>[2x]TSNFFCGEPIDYRGITAHRLVGAEPRPPVSGTRYAKVPGVPDEYKTGYRPANLGRSDPDSDKSLMNIAVKNLQVYQQEPKLDKVDEFIERAAADVLGYLRFLTKGERQANLNFKAAFNTLDLSTSCGPFVPGKKIDHVKDGVMDQVLAKHLYKCWSVANSGKALHHIYACGLKDELRPLDKVKEGKKRLLWGCDVGVAVCAAAVFHNICYKLKMVARFGPIAVGVDMTSRDVDVIINNLTSKASDFLCLDYSKWDSTMSPCVVRLAIDILADCCEQTELTKSVVLTLKSHPMTILDAMIVQTKRG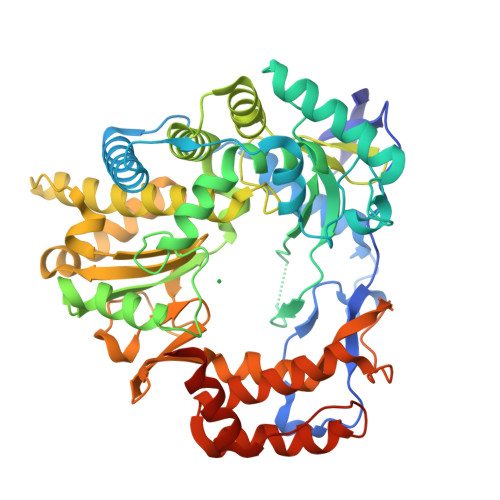LPSGMPFTSVINSICHWLLWSAAVYKSCAEIGLHCSNLYEDAPFYTYGDDGVYAMTPMMVSLLPAIIENLRDYGLSPTAADKTEFIDVCPLNKISFLKRTFELTDIGWVSKLDKSSILRQLEWSKTTSRHMVIEETYDLAKEERGVQLEELQVAAAAHGQEFFNFVCRELERQQAYTQFSVYSYDAARKILADRKRVVSVVPDDEFVNVME> MENTENSVDSKSIKNLEPKIIHGSESMDSGISLDNSYKMDYPEMGLCII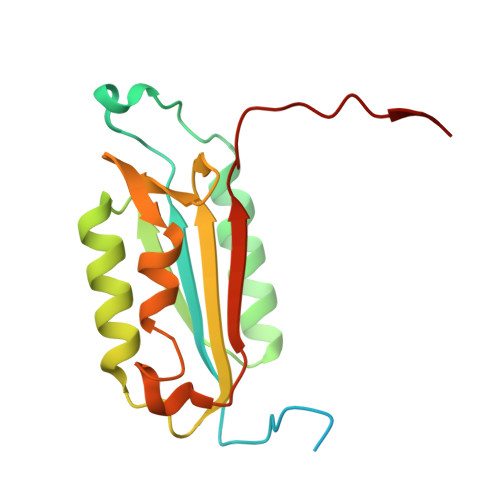INNKNFHKSTGMTSRSGTDVDAANLRETFRNLKYEVRNKNDLTREEIVELMRDVSKEDHSKRSSFVCVLLSHGEEGIIFGTNGPVDLKKITNFFRGDRCRSLTGKPKLFIIQACRGTELDCGIETD>AQSVPPGDINTQPGSKIVFNAPYDDKHTYHIKITNAGGRRIGWAIKTTNMRRLGVDPPSGVLDPSEKVLMAVSCDTFNAATEDLNNDR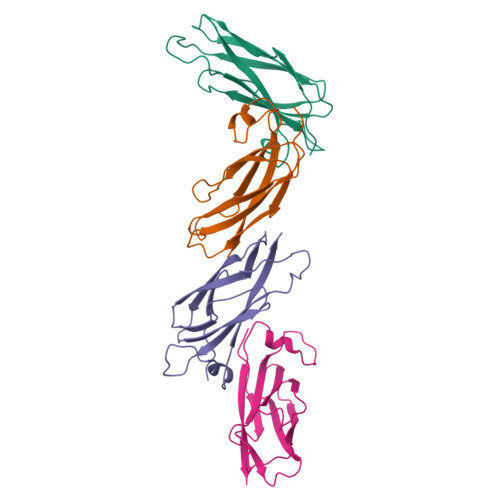ICIEWTNTPDGAAKQFRREWFQGDGMVRRKNLPIEYNL[8x]> MLAGRRPRREVLFFPSQVTCTEALLQAPGLPPGPSGCPCSLPHSESSLSRLLRALLAARSSLELCLFAFSSPQLGRAVQLLHQRGVRVRVITDCDYMALNGSQIGLLRKAGIQVRHDQDLG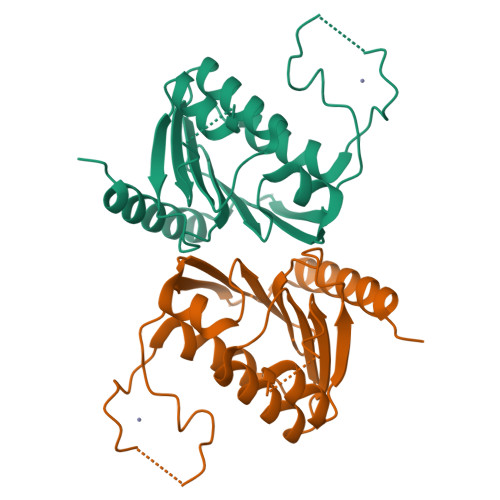YMHHKFAIVDKKVLITGSLNWTTQAIQNNRENVLIMEDTEYVRLFLEEFERIWEEFDPTKYSFFPQKHRGHLVPR>[5x]GVVELSADTSNQDLEEKLYNSILTGDYDSAVRQSLEYESQGKGSIIQNVVNNLIIDKRRNTMEYCYKLW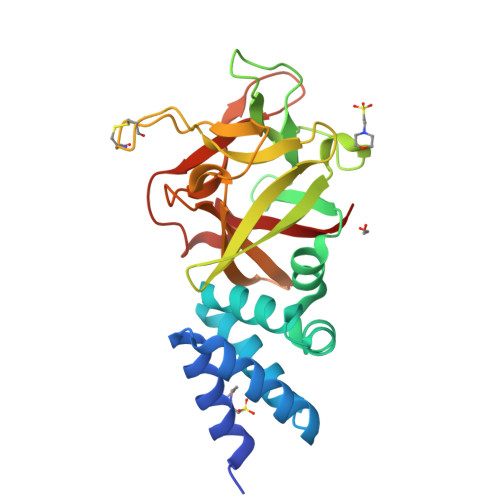VGNGQEIVRKYFPLNFRLIMAGNYVKIIYRNYNLALKLGSTTNPSNERIAYGDGVDKHTELVSWKFITLWENNRVYFKIHNTKYNQYLKMSTTTCNCNSRDRVVYGGNSADSTREQWFFQPAKYENDVLFFIYNRQFNDALELGTIVNASGDRKAVGHDGEVAGLPDIYSWFITPF> MSELTEAEKRRLLRERRQKKFSNGGASSR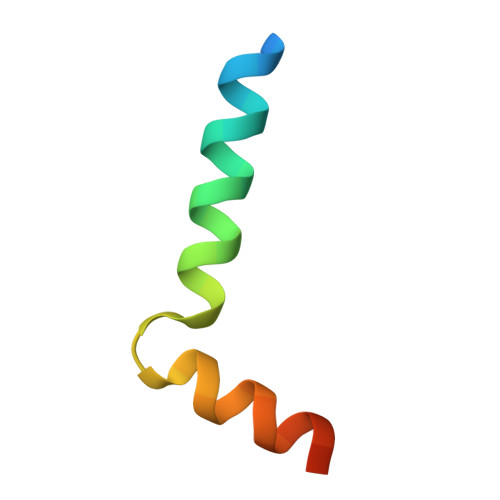LNKITGQAS> NQQKSLTLIVALTTSYGIGRSNSLPWKLKKEISYFKRVTSFVPTFDSFESMNVVLMGRKTWESIPLQFRPLKGRINVVITRNESLDLGNGIHSAKSLDHALELLYRTYGSESSVQINRIFVIGGAQLYKAAMDHPKLDRIMATIIYKDIHCDVF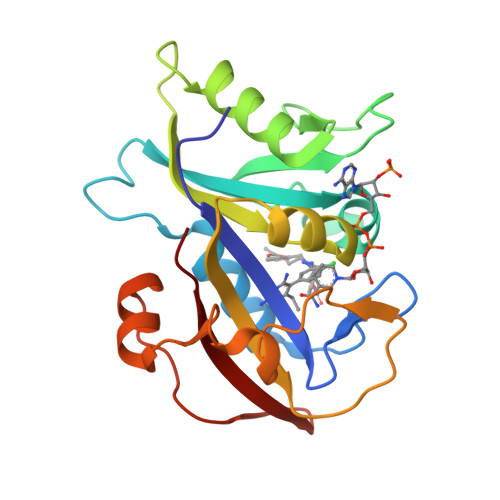FPLKFRDKEWSSVWKKEKHSDLESWVGTKVPHGKINEDGFDYEFEMWTRDL Protein translation relies on aminoacyl-tRNA synthetases (aaRSs) to charge tRNAs with their cognate amino acids. Plasmodium AspRS is a Class IIb aaRS that exhibits unusual sequence features compared with human AspRS, including initiation from an internal methionine, and an insert in the anticodon-binding domain. PvAspRS (96–631) was successfully crystallized as the apo protein, in complex with the natural intermediate, and with synthetic Asp-AMS and Asp-DACM, allowing insights into the binding determinants. As anticipated, PvAspRS adopts a dimeric structure with features typical of Type II aaRSs.

We solved the structure of apo PvAspRS and refined it to 2.1 Å resolution. In apo PvAspRS, residues SEGG of the Chain A flipping loop are not resolved. In Chain B, the flipping loop can be built. The SEGG loop interacts with a conserved residue Q371, as well as S350, N356 and A357. B-factor analysis suggests the SEGG loop is more mobile than neighboring regions of the protein. By contrast, in the equivalent region of apo PvAspRS (L347-Q371), the flipping loop and flanking β-hairpin are both well-defined in Chain B, while in apo Chain A, only the flipping loop itself is not resolved. By contrast, in apo PvAspRS, the equivalent region (R396-H405) is ordered. Interestingly, only minor shifts are observed after binding of ligands suggesting that the apo PvAspRS chain B flipping loop is poised to adopt a closed position. Thus, differences in the sequences of PvAspRS and EcAspRS in this region likely underpin the observed structural differences, enabling the apo PvAspRS chain B flipping loop to adopt a conformation that is poised to form a “closed” structure.

>AERENLKNEATKVLEHVCEDINKESYGFVKISKMKENEKEIRLFNLEEIYHSLMKVGGSGATDGGKREDDAASHSVVAESNGAHLLQSDIWVRGRIHDIRSKGSLAFIILRHKLYSMQCILDIKHNDNDKNMMKWVSNLPLESIVDIKGKLSKPEVPIDSTNIKYEAHIRKIFCISKTAKELPFLLKDANMKETNEEGSIKVNQDNRLNNRCVDLRTYANYSIFCLQSQICTIFKNFLLENNFIEIHTPKLLGESSEGGANAFQINYFNQKGFLAQSPQLYKQMCINSGFDRVFEVAPVFRAENSNTYRHLCEYVSLDVEMTYKYDYLENVHFYDSMFKHIFTELSKGGKNEMLIKTVKGQYPCEDFQWLEETPIFTYEEAIKMLIQHGKLHLKEEEILAYDMSTDMEKELGKIVKASHHTDYYIIINFPSALRPFYTMYKEDEPAISNSYDFFMRGEEILSGSQRISDVNLLLENIKRFNLDANKLNFYIDSFAYSSYPHSGCGIGLERVLMLFLGLNNIRKTSLFPRDPKRLIP[2x]> AQSVPWGISRVQAPAAHNRGLTGSGVKVAVLDTGISTHPDLNIRGGASFVPGEPSTQDGNGHGTHVAGTIAALNNSIGVLGVAPSAELYAVKVLGASGSGSVSSIAQGLEWAGNNGMHVANLSLGSPSPSATLEQAVNSATSRGVLVVAASGNSGAGSISYPARYANAMAVG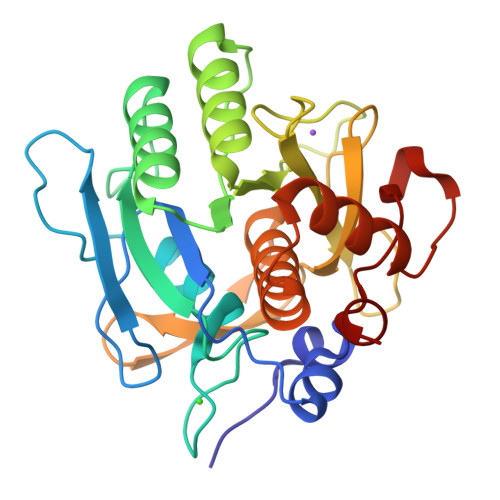ATDQNNNRASFSQYGAGLDIVAPGVNVQSTYPGSTYASLNGTSMATPHVAGAAALVKQKNPSWSNVQIRNHLKNTATSLGSTNLYGSGLVNAEAATR1-((4'-((6-amino-3H-purin-3-yl)methyl)biphenyl-4-yl)methyl)-4-(dimethylamino)pyridinium 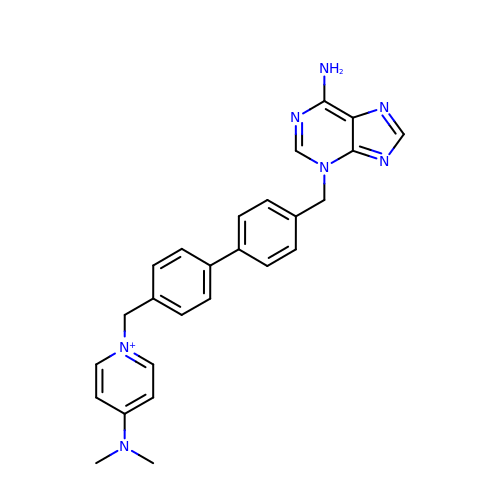| C26 H26 N7 | YZNBHTPOBJOYMF-UHFFFAOYSA-N> ASDQRGYKPEDVAFDESFFSFGGHVGTSVEYEDKVTRGFNNTDKKEKTITNEVFNFFYNNPQWNFMGFYSFKIENREQKEPGYYENEDGIKQLFSLNKGHDLGNGWATGLIYELEYTRSKVYSPDVSGLRKNLAEHSIRPYLTYWNNDYNMGFYSNLEYLLSKEDRNAWGKRQEQGYSALFKPYKRFGNWEVGVEFYYQIKTNDEKQPDGTINEKSDFNERYIEPIVQYSFDDAGTLYTRVRVGKNETKNTDRSGGGNAGINYFKDIRKATVGYEQSIGESWVAKAEYEYANEVEKKSRLSGWEARNKSELTQHT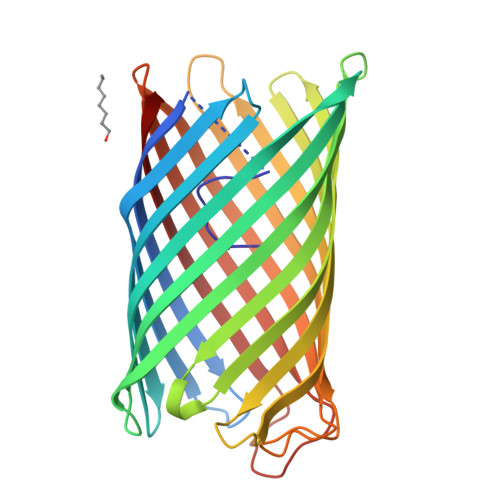FYAQALYRF>[3x]PLSVDSKTVNYFDIITIKHQDTDAFLHSHLARYPQRYEDGRI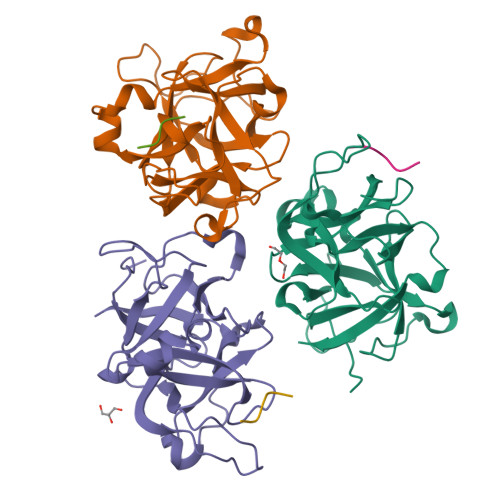SSAGQQVTGYTHPDFNNQWEVLPPHGSDVGKGQAVLLNQHIRLRHVATDTYLLAHDVASPFYPTNEEITTVTLEEGDGELYPETLFAFQPLKKSDEGHVLKSKTVSFRLFHVDTSVALWTHNDELLPDWGFQQQEINGNKKVIDPSNNWVVDEIVNLDEVRKVYIPKVV;>SSSASKTSTNATSSSCATPS[3x]>[4x]SMFSSTERHLTQKDPIMKPTIALIGRPNVGKSTLFNRLTRTKDALVHDLPGLTRDRHYGHGKVGSKPYFVIDTGGFEPVVDSGILHEMAKQTLQAVDEADAVVFLVDGRTGLTPQDKIIADRLRQSPRPVYLAVNKGEGGDRAVLAAEFYELALGEPHVISGAHGDGVYYLIEEILENFPEPEA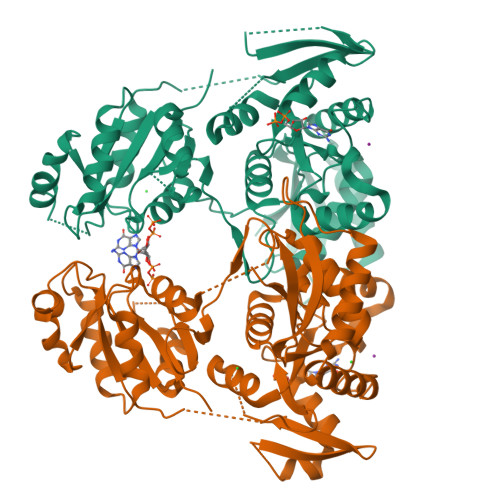EEADAKHPVFAVIGRPNVGKSTLVNAILGEKRVIAFDMAGTTRDSIHIDFEREGKPFTIIDTAGVRRRGKVDEAVEKFSVIKAMQAVEAANVAVLVLDAQQDIADQDATIAGFALEAGRALVVAVNKWDGISEERREQVKRDISRKLYFLDFAKFHFISALKERGIDGLFESIQAAYNAAMIKMPTPKITRVLQTAVGRQQPPRAGLVRPKMRYAHQGGMNPPVIVVHGNSLHAISDSYTRYLTQTFRKAFNLQGTPLRIQYNVSENPYENAED(5S,6S,9R,13R)-2,3-didehydro-5,6,7,8,9,10,11,12,13,14-decahydroretinoic acid | C20 H36 O2 | 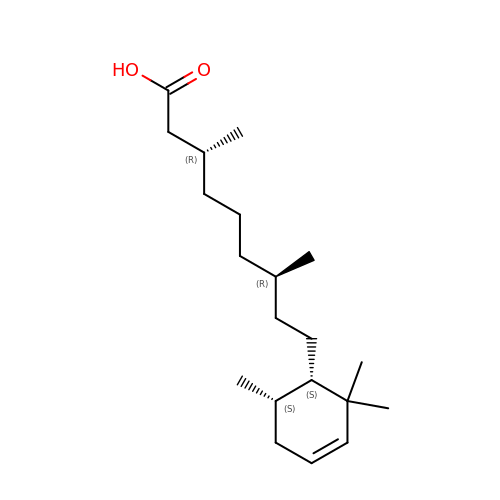IUMIJQXLDMMXRF-BDXSIMOUSA-N(1~{R},3~{S},5~{R})-~{N}2-(1-aminocarbonylindol-3-yl)-~{N}3-[3-(trifluoromethyloxy)phenyl]-2-azabicyclo[3.1.0]hexane-2,3-dicarboxamide 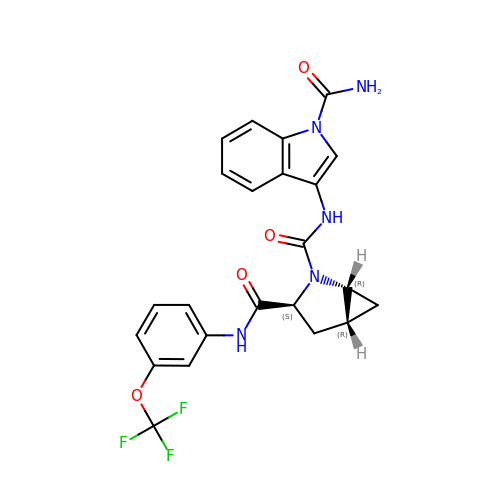| C23 H20 F3 N5 O4 | VERSLSAMPJEQIQ-DPMMWBKBSA-N5-[3,6-dihydro-2H-pyran-4-yl]-2-methoxy-N-[2-methylpyridin-4-yl]pyridine-3-sulfonamide 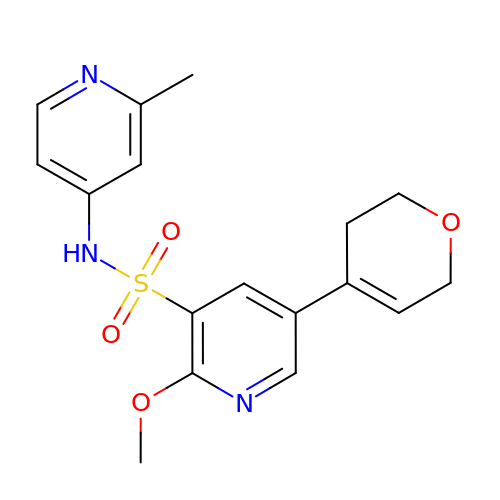| C17 H19 N3 O4 S | MQQOMKBMLHBDFG-UHFFFAOYSA-N> SMGPTSQRRGSLQLWQFLVALLDDPSNSHFIAWTGRGMEFKLIEPEEVARRWGIQKNRPAMNYDKLSRSLRYYYEKGIMQKVAGERYVYKFVCDPEALFSMAFSDN

The Ets transcription factor family consists of 28 genes in humans containing the evolutionarily conserved 85 amino acid Ets DNA-binding domain, originally identified as a viral oncogene (E26 transformation-specific). The Ets domain is a variant helix-turn-helix (winged helix) structure, comprising three α-helices and a four-stranded antiparallel β-sheet. Here, we present the crystal structures of the Ets domains of the entire PEA3 subfamily (Etv1, Etv4, and Etv5) together with the structure of the Erg family member (Fev). Furthermore, a new Ets dimerization interface linked by a redox-sensitive disulfide bond is identified, and this dimerization is shown to result in a significant inhibition of DNA binding, potentially linking Ets transcription factors with cellular redox regulatory mechanisms.

In all four DNA complexes, the recognition helix (α3) inserts deep into the major groove and provides multiple contacts with the base pairs of the core GGAA sequence, as well as with the phosphate backbone. Specifically in Etv1, hydrogen bonds to phosphate oxygens are formed with the side chains of residues Gln-336, Trp-375, Tyr-386, Ser-392, and Tyr-396, whereas salt bridges are formed with Lys-379, Lys-388, Lys-399, and Lys-404. Two additional charged residues, Arg-381 and Arg-409, appear to be in position with the potential to interact with the phosphodiester backbone; the former occupies a position between the two DNA strands in the region of the minor groove narrowing, and the latter could potentially form an additional salt bridge in longer DNA sequences. In both cases, the overall structure is very well conserved (root mean square deviation of ∼1 Å), with only minor movements of both the N and C termini and the β3-β4 loop, which appear to move away from the DNA in the DNA complexes of both Etv1 and Fev, avoiding potential steric overlaps that can be seen to occur following structural superposition. On an individual residue level, the most striking transitions can be seen to occur in the recognition helix α3, where in Etv1 Asp-387, Arg-391, and Arg-394 can be seen to become ordered upon DNA binding and Tyr-395, which can be seen to switch between the two alternative rotamers found to be important for recognition of bases downstream of the GGA motif in the Fev-DNA complex. Somewhat surprisingly, mutants in residues involved in salt bridges to the DNA backbone (Lys-379 and Lys-404) exhibited no detectable DNA binding. Overall, the mutational analysis demonstrates that the residues interacting with the DNA backbone in the crystal structure are the major contributors to the binding affinity in solution, although the interactions with the bases add a significant but lower energetic contribution. We were able to reproduce the inhibition of DNA binding by specific phosphorylation of Ser-334, a known PKA target site, in the isolated Ets domain in vitro.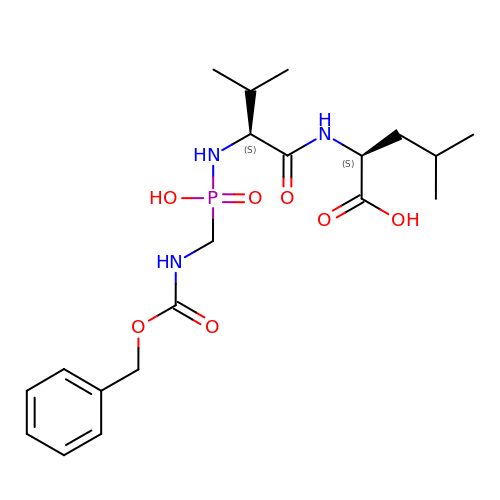N-[(S)-({[(benzyloxy)carbonyl]amino}methyl)(hydroxy)phosphoryl]-L-valyl-L-leucine | C20 H32 N3 O7 P | NFEZDCCCWWWKAJ-IRXDYDNUSA-N> MSQLQEMMTVVSQREVAYNIFEMVLKGTLVDEMDLPGQFLHLAVPNGAMLLRRPISISSWDKRAKTCTILYRIGDETTGTYKLSKLESGAKVDVMGPLGNGFPVAEVTSTDKILIIGGGIGVPPLYELAKQLEKTGCQMTILLG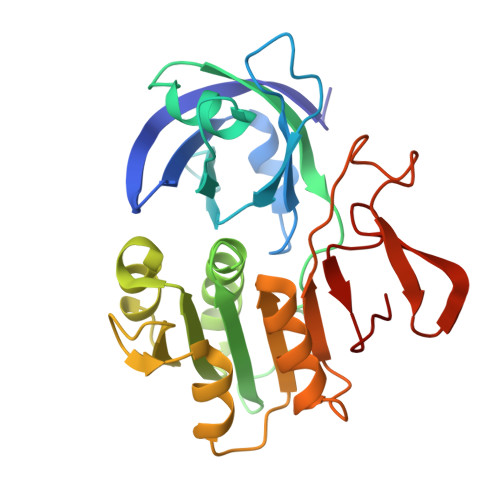FASENVKILENEFSNLKNVTLKIATDDGSYGTKGHVGMLMNEIDFEVDALYTCGAPAMLKAVAKKYDQLERLYISMESRMACGIGACYACVEHDKEDESHALKVCEDGPVFLGKQLSL> MDQWILGILGFVSTFLCLIGLLLVPVSANIEGDALNALKTNLADPN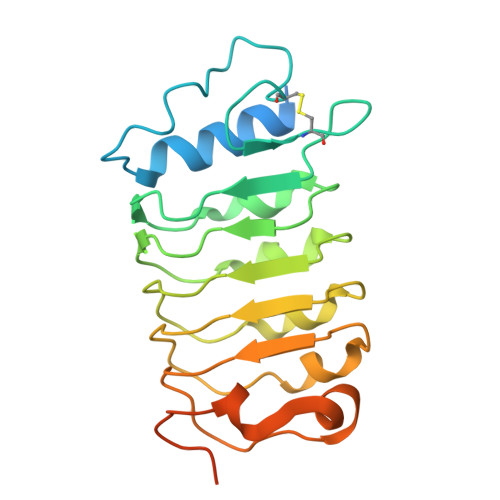NVLQSWDPTLVNPCTWFHVTCNSENSVTRVDLGNANLSGQLVPQLGQLPNLQYLELYSNNISGRIPFELGNLTNLVSLDLYLNRLNGPIPDTLGKLQKLRFLRLNNNSLNGRIPMLLTTVISLQVLDLSNNNLTGPVPVNGSFSLFTPISFANNPLDIPPAAPPPPISPMPPSSSGVGNSAT> GSVHKHTGRNCGRKFKIGEPLYRCHECGCDDTCVLCIHCFNPKDHVNHHVCTDICTEFTSGICDCGDE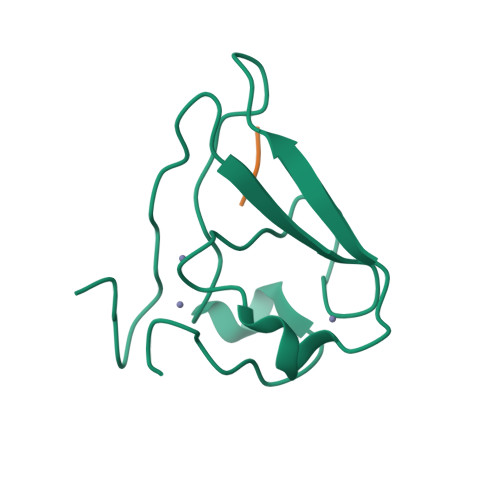EAWNSPLHCKAEEQ;> KIAA> MSDGAVQPDGGQPAVRNERATGSGNGSGGGGGGGSGGVGISTGTFNNQTEFKFLENGWVEITANSSRLVHLNMPESENYRRVVVNNMDKTAVNGNMALDDIHAQIVTPWSLVDANAWGVWFNPGDWQLIVNTMSELHLVSFEQEIFNVVLKTVSESATQPPTKVYNNDLTASLMVALDSNNTMPFTPAAMRSETLGFYPWKPTIPTPWRYYFQWDRTLIPSHTGTSGTPTNIYHGTDPDDVQFYTIENSVPVHLLRTGDEFATGTFFFDCKPCRLTHTWQTNRALGLPPFLNSLPQSEGATNFGDIGVQQDKRRGVTQMGNTNYITEATIMRPAEVGYSAPYYSFEASTQGPFKTPIAAGRGGAQTDENQAADGNPRYAFGRQHGQKTTTTGETPERFTYIAHQDTGRYPEGDWIQNINFNLPVTNDNVLLPTDPIGGKTGINYTNIFNTYGPLTALNNVPPVYPNGQIWDKEFDTDLKPRLHVNAPFVCQNNCPGQLFVKVAPNLTNEYDPDASANMSRIVTYSDFWWKGKLVFKAKLRASHTWNP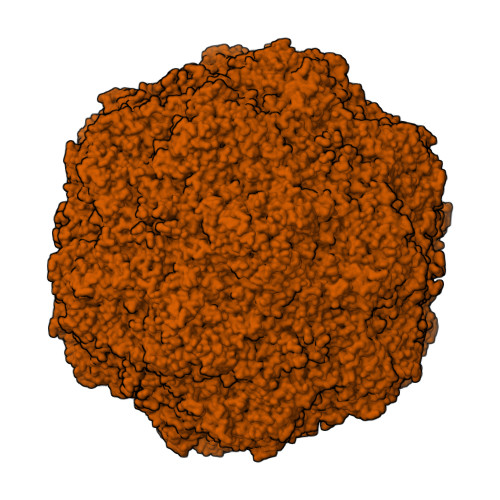IQQMSINVDNQFNYVPSNIGGMKIVYEKSQLAPRKLY> LSEQLKHCNGILKELLSKKHAAYAWPFYKPVDASALGLHDYHDIIKHPMDLSTVKRKMENRDYRDAQEFAADVRLMFSNCYKYNPPDHDVVAMARKLQDVFEF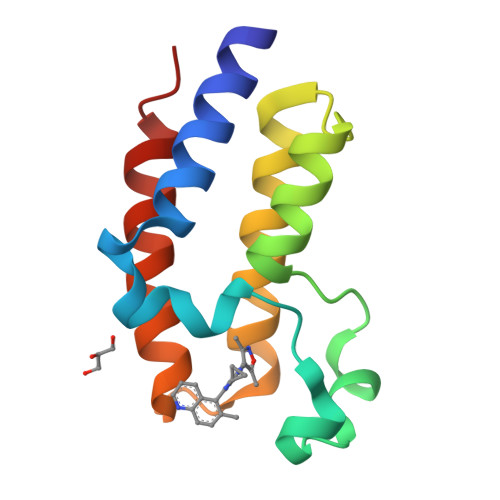RYAKMPD> NKSLVDQMLVELDKKISAQMDEILHNSQFQAMESAWRGLKLFVDRTDFRENNKVEILHVTKDELLEDFEFAPETAQSGLYKHVYSAGYGQFGGEPVGAIIGNYAFTPSTPDMKLLQYMGALGAMAHAPFISSVGPEFFGIDSFEELPNIKDLKSTFESPKYTKWRSLRESEDARYLGLTAPRFLLRVPYDPIENPVKSFNYAENVSASHEHYLWGNTAFAFATRLTDSFAKYRWCPNIIGPQSGGAVEDLPVHVFES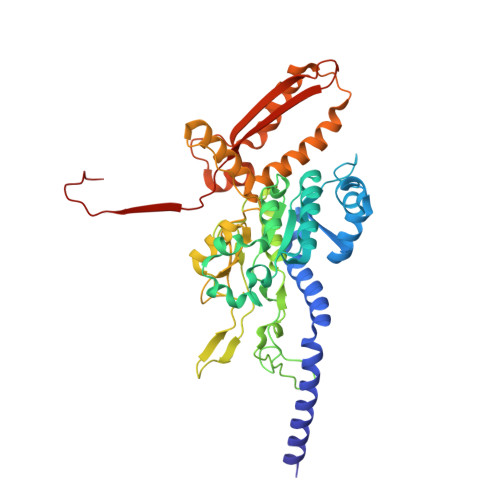MGALQSKIPTEVLITDRKEFELAEEGFIALTMRKGSDNAAFFSANSIQKPKVFPNTKEGKEAETNYKLGTQLPYMMIINRLAHYVKVLQREQIGAWKERQDLERELNSWIKQYVADQENPPADVRSRRPLRAARIEVMDVEGNPGWYQVSLSVRPHFKYMGANFELSLVGRLDQA> SNASVERVYQKKTQLEHILLRPDTYIGSVEPLTQFMWVYDEDVGMNCREVTFVPGLYKIFDEILVNAADNKQRDKNMTCIKVSIDPESNIISIWNNGKGIPVVEHKVEKVYVPALIFGQLLTSSNYDDDEKKVTGGRNGYGAKLCNIFSTKFTVETAC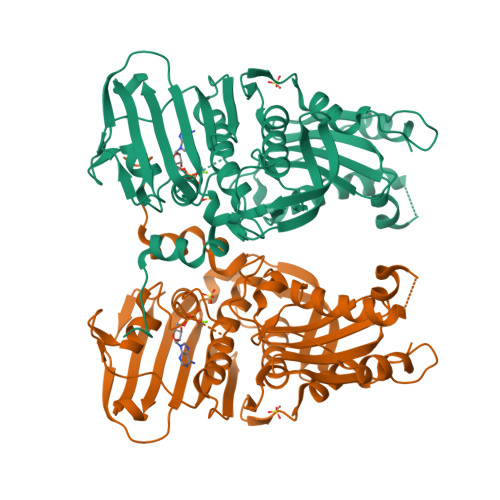KEYKHSFKQTWMNNMMKTSEAKIKHFDGEDYTCITFQPDLSKFKMEKLDKDIVALMTRRAYDLAGSCRGVKVMFNGKKLPVNGFRSYVDLYVKDKLDETGVALKVIHELANERWDVCLTLSEKGFQQISFVNSIATTKGGRHVDYVVDQVVGKLIEVVKKKNKAGVSVKPFQVKNHIWVFINCLIENPTFDSQTKENMTLQPKSFGSKCQLSEKFFKAASNCGIVESILNWVKFKAQTQLNKKCS>[2x]EDADKLPHTKVTLVAPPQVHPHEQATKSGPKVVEFTMTIEEKKMVIDDKGTTLQAMTFNGSMPGPTLVVHEGDYVQLTLVNPATNAMPHSVDFHGATGALGGAKLTNVNPGEQATLRFKADRSGTFVYHCAPEGMVPWHVVSGMS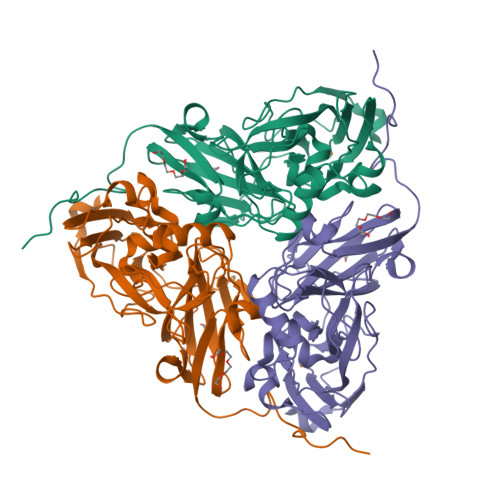GTLMVLPRDGLKDPQGKPLHYDRAYTIGEFDLYIPKGPDGKYKDYATLAESYGDTVQVMRTLTPSHIVFNGKVGALTGANALTAKVGETVLLIHSQANRDTRPHLIGGFGDWVWETGKFANPPQRDLETWFIRGGSAGAALYTFKQPGVYAYLNHNLIEAFELGAAGHIKVEGKWNDDLMKQIKAPAPIPR> MEIETVEVAPQQEEEFKLDYDLLEEYYRSYFPVS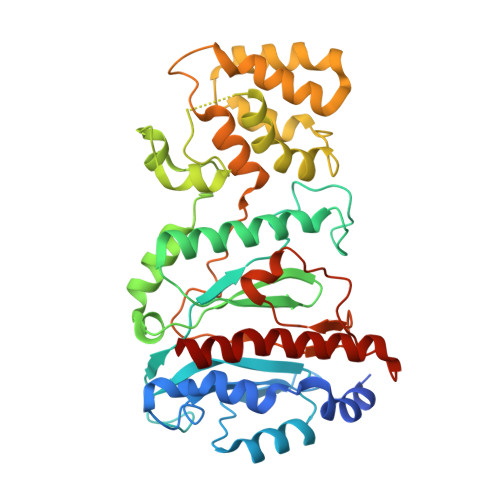QMVQWLSYPQDGDDTYFTRREFSFTLQNEVYLRYQMYNSEREFKNALLQKVPEKIDIGAVYDRPGKKGDDIKAKEKEFVIDIDMTDYDHIRTCCSKAKICEKCWKFMRVACDLISKSLDEDFGFQHVLWVYSGRRGIHAWVCDKEIRKANDYTRASIIDYLNILVDNSIGSSYVKPSLLKMEKSHLIERNAMKQLNQKNDDLKAEKESEKVFVEIVLREQNLFMKKPEIILEFLAKRSENLSKEVEKEWKTLKTSEQRYEALKELVSSEDKKKTHYLLEELRIWLLYPRLDVNVSKSTNHLLKSPFCIHPKTGNVCVPFTTEEISTFDPFSVPNISTLTTEEGSSKMKNSLKIFNKFLENLKKDV> QDAASGEQVFKQCLVCHSIGPGAKNKVGPVLNGLFGRHSGTIEGFAYSDANKNSGITWTEEVFREYIRDPKAKI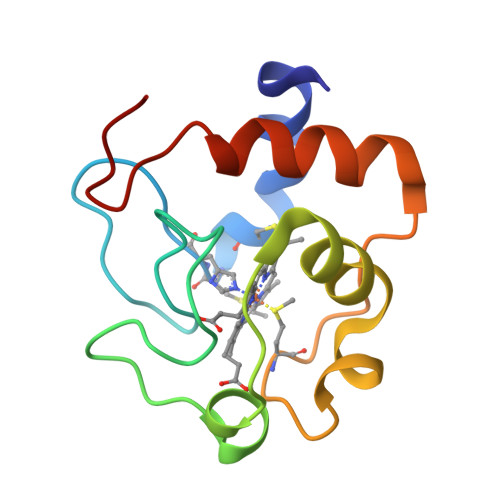PGTKMIFAGVKDEQKVSDLIAYIKQFNADGSKK> SNMWVIGKSKAQDAKAIMVNGPQFGWYAPAYTYGIGLHGAGYDVTGNTPFAYPGLVFGHNGVISWGSTAGFGDDVDIFAERLSAEKPGYYLHNGKWVKMLSREETITVKNGQAETFTVWRTVHGNILQTDQTTQTAYAKSRAWDGKELASLLAWTHQMKAKNWQEWTQQAAKQALTINWYYADVNGNIGYVHTGAYPDRQSGHDPRLPVPGTGKWDWKGLLPFEMNPKVYNPQSGYIANWANSPQKDYPASDLFAFLWGGADRVTEIDRLLEQKPRLTADQAWDVIRQTSRQDLNLRLFLPTLQAATSGLTQSDPRRQLVETLTRWDGINLLNDDGKTWQQPGSAILNVWLTSMLKRTVVAAVPMPFDKWYSASGYETTQDGPTGSLNISVGAKILYEAVQGDKSPIPQAVDLFAGKPQQEVVLAALEDTWETLSKRYGNNVSNWKTPAMALTF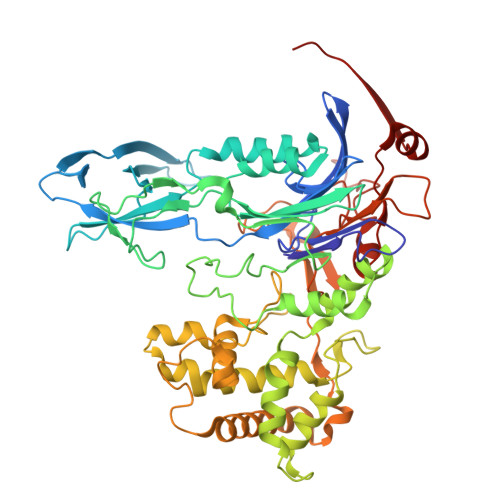RANNFFGVPQAAAEETRHQAEYQNRGTENDMIVFSPTTSDRPVLAWDVVAPGQSGFIAPDGTVDKHYEDQLKMYENFGRKSLWLTKQDVEAHKESQEVLHVQR>[2x]RTETDFSNLFARDLLPAKNGEEQTVQFLLEVVDILLNYVRKTFDRSTKVLDFHHPHQLLEGMEGFNLELSDHPESLEQILVDCRDTLKYGVRTGHPRFFNQLSTGLDIIG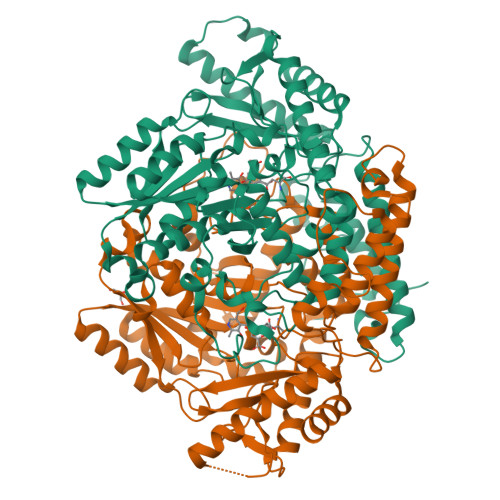LAGEWLTSTANTNMFTYEIAPVFVLMEQITLKKMREIVGWSSKDGDGIFSPGGAISNMYSIMAARYKYFPEVKTKGMAAVPKLVLFTSEQSHYSIKKAGAALGFGTDNVILIKCNERGKIIPADFEAKILEAKQKGYVPFYVNATAGTTVYGAFDPIQEIADICEKYNLWLHVDAAWGGGLLMSRKHRHKLNGIERANSVTWNPHKMMGVLLQCSAILVKEKGILQGCNQMHASYLFQQDKHYDVSYDTGDKAIQCGRHVDIFKFWLMWKAKGTVGFENQINKCLELAEYLYAKIKNREEFEMVFNGEPEHTNVCFWYIPQSLRGVPDSPQRREKLHKVAPKIKALMMESGTTMVGYQPQGDKANFFRMVISNPAATQSDIDFLIEEIERLGQDLHHHHHH> MAHHHHHHMSKKRVLTGVTTTGTPHLGNYVGAIRPAVRAAQNPDTESFLFLADYHGIIKCHEQEMIHQSTQAVAATWLACGLDPERTTFYRQSDIPEVMELNWILTCIT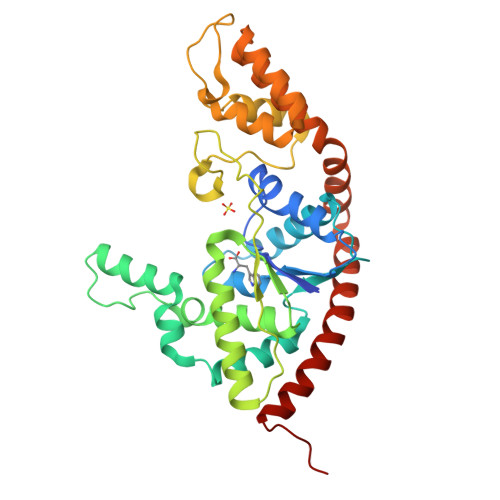AKGLMNRAHAYKAAVQANAENGQEDPDFGVEMGLFSYPILMTADILMFNANEVPVGRDQIQHVEMARDIAGRFNHRFQELFTLPEVKIDENVELLVGLDGRKMSKSYGNTIPLWENDKKTQKSVNKIITNMKEPGEPKQPDESPLFEIYKAFSTPSETAEFTQMLADGLAWGEAKKLSAAKINAELAELRERYNALTSNPSQIEEILQAGAQKARKEARELLDKVRDAVGIRPLK>MNTTLFRWPVRVYYEDTDAGGVVYHASYVAFYERARTEMLRHHHF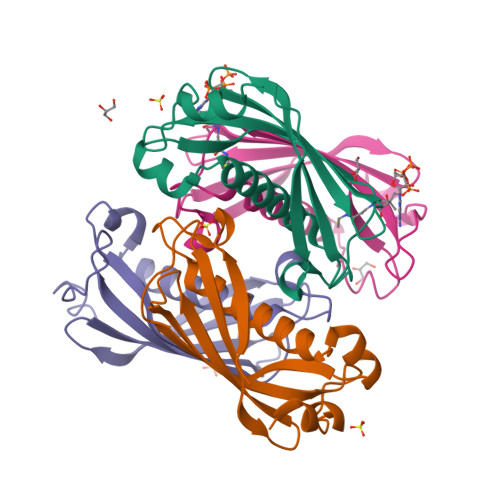SQQALMAERVAFVVRKMTVEYYAPARLDDMLEIQTEITSMRGTSLVFTQRIVNAENTLLNEAEVLVVCVDPLKMKPRALPKSIVAEFKQ[4x]> MPNFSGNWKIIRSENFEELLKVLGVNVMLRKIAVAAASKPAVEIKQEGDTFYIKTSTTVRTTEINFKVGEEFEEQTVDGRPCKSLVKWESENKMVCEQKLLKGEGPKTSWTRELTNDGELILTMTADDVVCTRVYVRE

The cellular retinoic acid-binding proteins CRABPI and CRABPII act as gatekeepers and facilitators for the passage of all-trans-retinoic acid (and related derivatives) through the cytoplasm to access retinoic acid receptors (RARs) in the nucleus. In this article, crystal structures are presented of the L29C mutant of Homo sapiens CRABPI in complex with naturally occurring fatty acids (1.64 Å resolution) and with the synthetic retinoid DC645 (2.41 Å resolution), and of CRABPII in complex with the ligands DC479 (1.80 Å resolution) and DC645 (1.71 Å resolution). The retinoic acid-binding ability of both CRABPI and CRABPII is centred on a hydrophobic pocket created by an orthogonal β-sheet fold and capped with a pair of antiparallel α-helices formed from residues 15–35 partway into the sequence. The pocket contains, at its most buried end, a trio of residues (Arg112, Arg132 and Tyr134 in CRABPI; Arg112, Arg133 and Tyr135 in CRABPII) that are responsible for binding to the carboxylic acid moiety of ATRA, usually in concert with a water molecule that is conserved in all structures with similarly binding ligands.

DC645 was developed as part of a library of synthetic retinoids following the EC23 archetype but lacking the fluorescence-enhancing elements used in earlier series (including DC479). Instead, a tetrahydroquinoxaline derivative offers enhanced hydrogen-bonding opportunities in the mid-section, creating interactions with solvent and Arg60 at the mouth of the binding site, which is likely to help to stabilize the protein–ligand complex. DC645 was chosen for co-crystallization owing to the increasing evidence of its positive effect on neurite outgrowth in cellular models of Alzheimer’s disease. The incorporation of DC645 into the CRABPII binding site, fully engaged with the binding triad, is an important step in understanding its interaction with the retinoid signalling pathway and indicates that the molecule will be transported to the nucleus. The ligand-binding residues and the carboxylic acid motif of the ligand are very closely aligned, with a slight deviation of the tetrahydroquinoxaline tail groups between the CRABPI-L29C and CRABPII structures. The structures presented above may also offer some insight into why CRABPII binds DC645 with greater efficacy than CRABPI-L29C. It can be seen in the ligand-binding site that residue Arg60, which is positioned to create a hydrogen-bonding network between the ligand and several water molecules in CRABPII, does not have the same orientation relative to the ligand in CRABPI-L29C.> MENFPIISLDKVNGVERAATMEMIKDACENWGFFELVNHGIPREVMDTVEK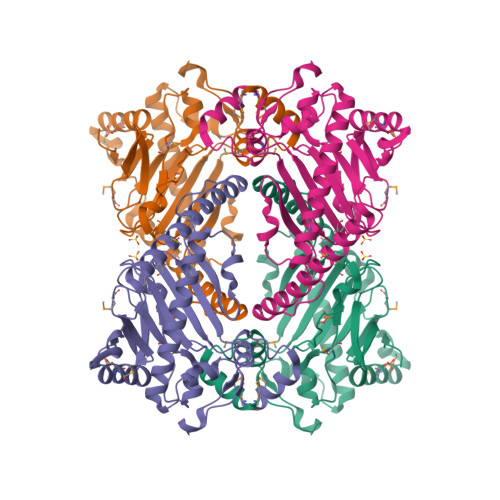MTKGHYKKCMEQRFKELVASKALEGVQAEVTDMDWESTFFLKHLPISNISEVPDLDEEYREVMRDFAKRLEKLAEELLDLLCENLGLEKGYLKNAFYGSKGPNFGTKVSNYPPCPKPDLIKGLRAHTDAGGIILLFQDDKVSGLQLLKDGQWIDVPPMRHSIVVNLGDQLEVITNGKYKSVMHRVIAQKDGARMSLASFYNPGSDAVIYPAPALVEKEAEENKQVYPKFVFDDYMKLYAGLKFQAKEPRFEAMKAMETDVKMDPIATV>[2x]MERKHHFVLVHNACHGAWIWYKLKPLLESAGHRVTAVELAASGIDPRPIQAVETVDEYSKPLIETLKSLPENEEVILVGFSFGGINIALAADIFPAKIKVLVFLNAFLPDTTHVPSHVLDKLMEMFGGW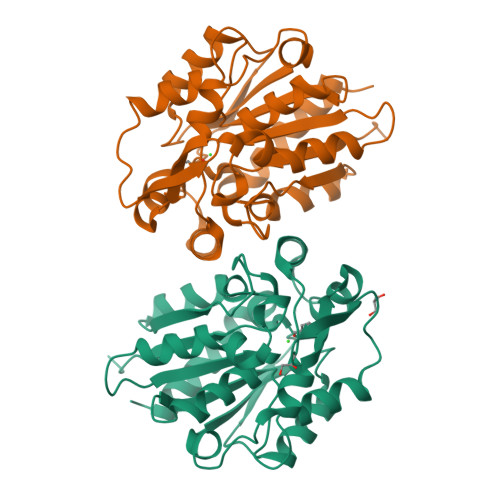GDTEFSSHETRNGTMSLLKMGPKFMKARLYQNCPIEDYELAKMLHRQGSFFTEDLSKKEKFSEEGYGSVQRVYVMSSEDKIIPCDFIRWMIDNFNVSKVYEIDGGDHMVMLSKPQKLFDSLSAIATDYMGL> TEFKAGSAKKGATLFKTRCLQCHTVEKGGPHKVGPNLHGIFGRHSGQAEGYSYTDAIIKKNVLWDENNMSEYLTNPKK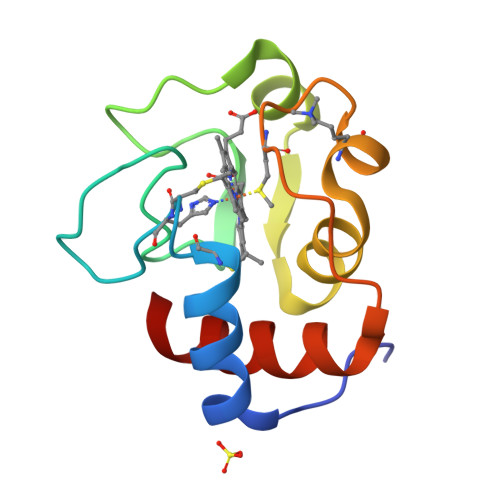YIPGTKMAFGGLKKEKDRNDLITYLKKATE>MARRILVVEDEAPIREMVCFVLEQNGFQPVEAE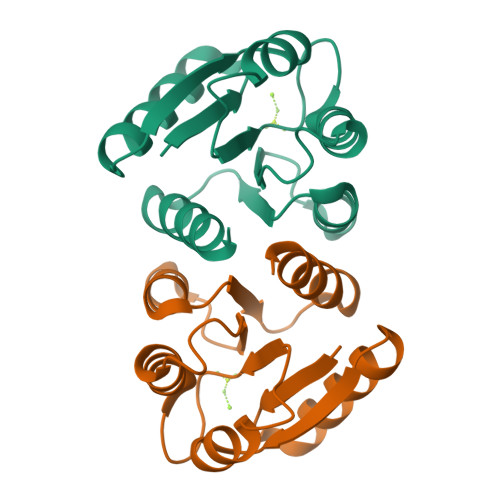DYDSAVNQLNEPWPDLILLDWMLPGGSGIQFIKHLKRESMTRDIPVVMLTARGEEEDRVRGLETGADDYITKPFSPKELVARIKAVMRRISQ[3x]>MTSNLQADMPLERIIEAEKRVECNDPLVALVVNENNTTVNNICQATHKQLFQLVQWAKLVPHFTSLPLTDQVQLLRAGWNELLIAAFSHRSMQAQDAIVLATGLTVNKSTAHAVGVGNIYDRVLSELVNKMKEMKMDKTELGCLRAIILYNPDVRGIKSVQEVEMLREKIYGVLEEYTRTTHPNEPGRFAKLLLRLPALRSIGLKCLEHLFFFKLIGDVPIDTFLMEMLEGTTDS[4x];>GSHMNGSKGISPEQEELIHRLVYFQNEYEHPSEEDVKRIINQPMDGEDQCDVRFRHITEITILTVQLIVEFAKRLPGFDKLLR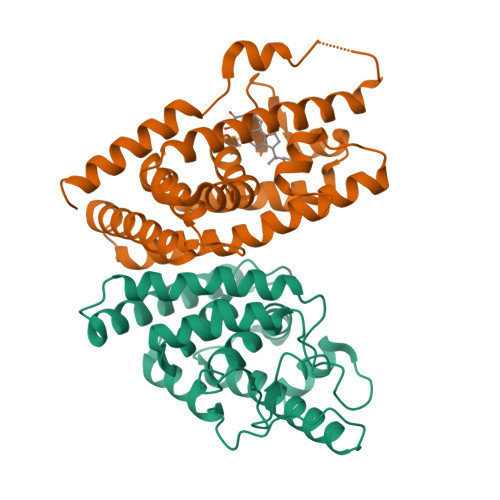EDQIALLKACSSEVMMFRMARRYDVQTDSILFVNNQPYSRDSYNLAGMGETIEDLLHFCRTMYSMRVDNAEYALLTAIVIFSERPALIEGWKVEKIQEIYLEALRAYVDNRRKPKPGTIFAKLLSVLTELRTLGNQNSEMCFSLKLKNKKLPPFLAEIWDVDLKT[4x]>SMAPWGKRLAGVRGVLLDISGVLYDSGAGGGTAIAGSVEAVARLKRSRLKVRFCTNESAASRAELVGQLQRLGFDISEQEVTAPAPAACQILKERGLRPYLLIHDGVRSEFDQIDTSNPNCVVIADAGESFSYQNMNNAFQVLMELEKPVLISLGKGRYYAATSGLMLDVGPYMKALEYACGIKAEVVGKPSPEFFKSALQAIGVEAHQAVMIGDDIVGDVGGAQRCGMRALQVRTGKFRPSDEHHPEVKA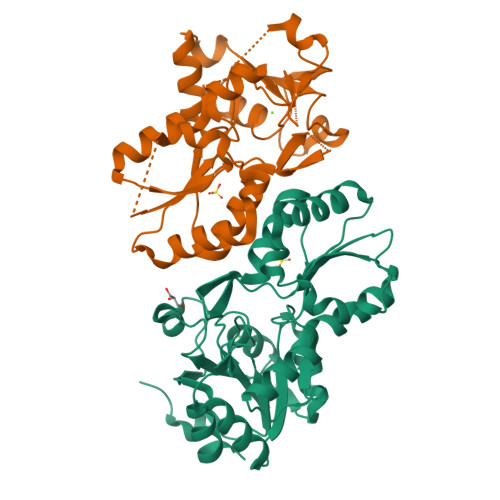DGYVDNLAEAVDLLLQHADK[2x]>AATYAQTLQNIPETNVTTLDNGLRVASEESSQPTCTVGVWIGAGSRYENEKNNGAGYFVEHLAFKGTKKRPCAAFEKEVESMGAHFNGYTSREQTAFYIKALSKDMPKVVELLADVVQNCALEESQIEKERGVILQELKEMDNDMTNVTFDYLHATAFQGTALARTVEGTTENIKHLTRADLASYIDTHFKAPRMVLAAAGGISHKELVDAARQHFSGVSFTYKEDAVPILPRCRFTGSEIRARDDALPVAHVALAVEGPGWADPDNVVLHVANAIIGRYDRTFGGGKHLSSRLAALAVEHKLCHSFQTFNTSYSDTGLFGFHFVADPLSIDDMMFCAQGEWMRLCTSTTESEVKRAKNHLRSAMVAQLDGTTPVCETIGSHLLNYGRRISLEEWDSRISAVDARMVRDVCSKYIYDKCPALAAVGPIEQLLDYNRIRSGMYWIRF[2x];>[2x]SLKVAPKVAVSAAAERVKLCPGAEDLEITKLPNGLIIASLENFSPASRIGVFIKAGSRYETTANLGTAHLLRLASPLTTKGASSFRITRGIEAVGGSLSVYSTREKMTYCVECLRDHVDTVMEYLLNVTTAPEFRPWEVTDLQPQLKVDKAVAFQSPQVGVLENLHAAAYKTALANPLYCPDYRIGKITSEQLHHFVQNNFTSARMALVGIGVKHSDLKQVAEQFLNIRSGAGTSSAKATYWGGEIREQNGHSLVHAAVVTEGAAVGSAEANAFSVLQHVLGAGPLIKRGSSVTSKLYQGVAKATTQPFDASAFNVNYSDSGLFGFYTISQAAHAGEVIRAAMNQLKAAAQGGVTEEDVTKAKNQLKATYLMSVETAQGLLNEIGSEALLSGTHTAPSVVAQKIDSVTSADVVNAAKKFVSGKKSMAASGDLGSTPFLDEL;>MAPNIRKSHPLLKMINNSLIDLPAPSNISAWWNFGSLLAVCLMTQILTGLLLAMHYTADTSLAFSSVAHTCRNVQYGWLIRNLHANGASFFFICIFLHIGRGLYYGSYLYKETWNTGVILLLTLMATAFVGYVLPWGQMSFWGATVITNLFSAIPYIGHTLVEWAWGGFSVDNPTLTRFFALHFLLPFAIAGITIIHLTFLHESGSNNPLGISSDSDKIPFHPYYSFKDILGLTLMLTPFLTLALFSPNLLGDPENFTPANPLVTPPHIKPEWYFLFAYAILRSIPNKLGGVLALAASVLILFLIPFLHKSKQRTMTFRPLSQTLFWLLVANLLILTWIGSQPVEHPFIIIGQMASLSYFTILLILFPTIGTLENKMLNY[2x];>GELELHPPAFPWSHGGPLSALDHSSVRRGFQVYKQVCSACHSMDYVAFRNLIGVTHTEAEAKALAEEVEVQDGPDENGELFMRPGKISDYFPKPYPNPEAARAANNGALPPDLSYIVNARHGGEDYVFSLLTGYCDPPAGVVVREGLHYNPYFPGQAIGMAPPIYNEILEYDDGTPATMSQIAKDVCTFLRWAAEPEHDQRKRMGLKMLLISALLTSLLYYMKRHKWSVLKSRKMAYRPPK[2x];>VHNDVTVPDFSAYRREDVMDATTSSQTSSEDRKGFSYLVTATACVATAYAAKNVVTQFISSLSASADVLALSKIEIKLSDIPEGKNVAFKWRGKPLFVRHRTQAEINQEAEVDVSKLRDPQHDLDRVKKPEWVILVGVCTHLGCVPIANSGDFGGYYCPCHGSHYDASGRIRKGPAPYNLEVPTYQFVGDDLVVVG[2x];>AARATVAGGGRLMDRIRKWYYNAAGFNKYGLMRDDTLYEDDDVKEALKRLPKDLYNERMFRIKRALDLSLKHRILPKEQWVKYEEDKPYLEPYLKEVIRERLEREAWNKK[2x];>GIHFGNLARVRHIITYSLSPFEQRAIPNIFSDALPNVWRRFSSQVFKVAPPFLGAYLLYSWGTQEFERLKRKNPADYENDQ[2x];>LRGSGEEEEEELVDPLTTIREHCEQTEKCVKARERLELCDARVSSRSHTEEQCTEELFDFLHARDHCVAHKLFNKLK[2x];>[2x]ALLRQAYSALFRRTSTFALTVVLGAVLFERAFDQGADAI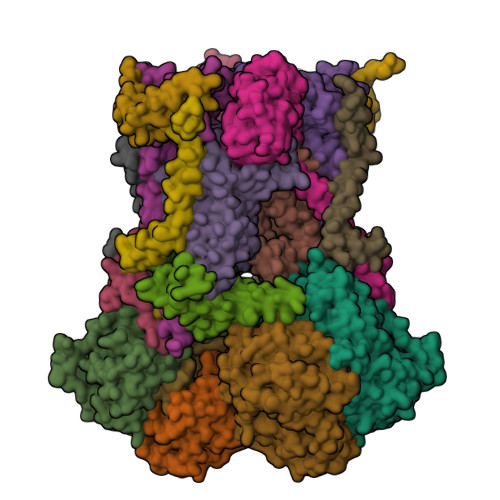FEHLNEGKLWKHIKHKYEASEE>MENSLFNQEVQIPLTESYCGPCPKNWICYKNNCYQFFDESKNWYESQASCMSQNASLLKVYSKEDQDLLKLVKSYHWMGLVHIPTNGSWQWEDGSILSPNLLTIIEMQKGDCALYASSFKGYIENCSTPNTYICMQRTV[2x];> MEPHSLRYNLTVLSWDGSVQSGFLTEVHLDGQPFLRCDRQKCRAKPQGQWAEDVLGNKTWDRETRDLTGNGKDLRMTLAHIKDQKEGLHSLQEIRVCEIHEDNSTRSSHHFYYDGELFLSWNLETKEFTMPQSSRAQTLAMNVRNFWKEDAMKTKTHFHAMHADCLQELRRYLKSGVVLRRTVPPMVNVTRSEASEGNITVTCRASGFYPWNITLSWRQDGVSLSHDTQQWGDVLPDGNGTYQTWVAT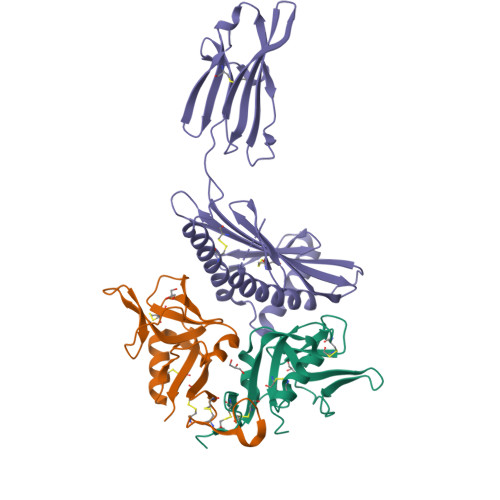RICQGEEQRFTCYMEHSGNHSTHPVPS>MLYAQVNGINLHYEIEGQGQPLLLIMGLGAPAAAWDPIFVQTLTKTHQVIIYDNRGTGLSDKPDMPYSIAMFASDAVGLLDALNIPRAHVFGVSMGGMIAQELAIHYPQRVASLILGCTTPGGKHAVPAPPESLKALEGRAGLTPEEAIREGWKLSFSEEFIHTHKAELEAHIPRLLAQLTPRFAYERHFQATMTLRVFKQLKEIQAPTLVATGRDDMLIPAVNSEILAREIPGAELAIFESAGHG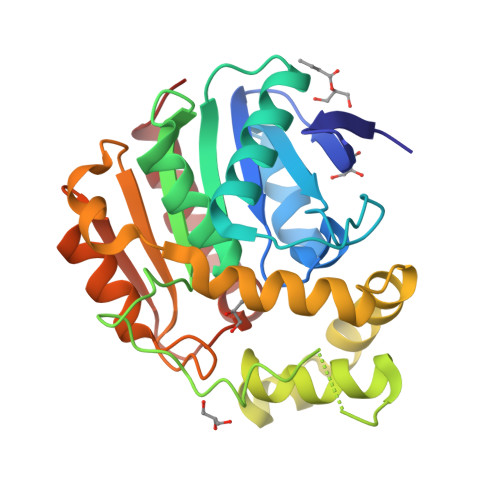FVTSAREPFLKVLKEFLARQSV[4x]> MEEEAETEEQQRFSYQQRLKAAVHYTVGCLCEEVALDKEMQFSKQTIAAISELTFRQCENFAKDLEMFARHAKRTTINTEDVKLLARRSNSLLKYITDKSEEIAQINLERKAQKKKKSEDGSKNSRQPAEAGVVESE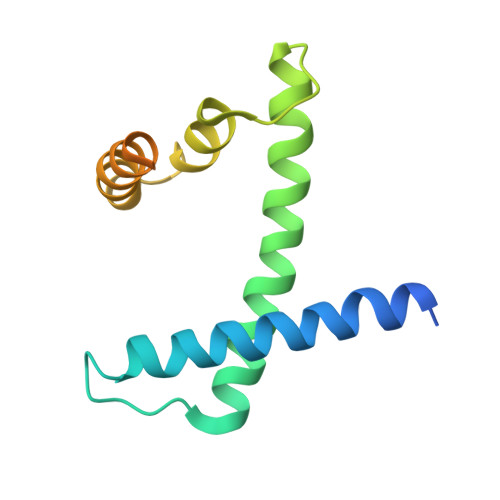N>HGFVDSPGARNYFCGAVTKPDHVMNGVARYPECAGAFANDFNGGYSYMSVLTHHQGRKVLGPVARNVCGFDSETWNGGKTPWDNAINWPVNNINSGTLTFSWDISNGPHFDDTSDFRYWITKPGFVYQVGRELTWADFEDQPFCDLAYNDDNPGAYPNVRADKPNTHFHTTCTVPARTGRHVIYAEWGREPPTYE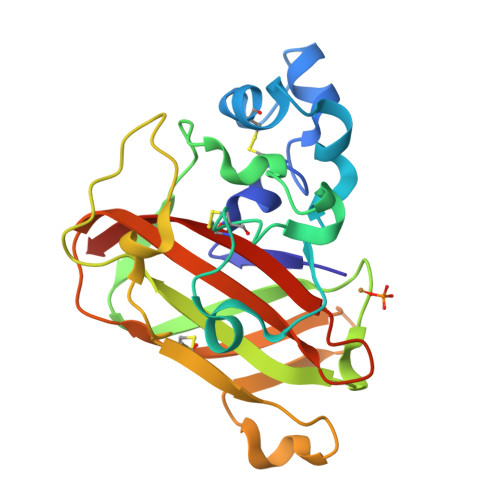RFHGCIDVQIHHHHHH[8x]Dihydrofolate reductase (DHFR) is a key and essential enzyme in the folate pathway that converts dihydrofolate (DHF) to tetrahydrofolate (THF) (Raimondi et al., 2019). This coenzyme is required for a variety of cellular processes, including the synthesis of purine involved in nucleic acid and amino-acid biosynthesis. The active site is located in a cleft formed by α-helix 1, α-helix 2, α-helix 4 and β-sheet 1, similar to CglDHFR and CalDHFR. As classified in E. coli DHFR, CauDHFR could also be designated to have two subdomains: the nucleotide subdomain, in which the NADPH sits, and the substrate-binding subdomain, which is predominantly formed by α-helix 1, α-helix 2 and β-sheet 1.

Crystals of apo and holo CauDHFR have a single protomer in the asymmetric unit, while the ternary complexes CauDHFR–NADPH–PYR and CauDHFR–NADPH–CYG contained two protein molecules which are independent and do not form a quaternary structure, according to the PISA server. In order to obtain the structures of the CauDHFR–NADPH–PYR and CauDHFR–NADPH–CYG ternary complexes, the N-terminal His tag of the protein needed to be removed since analysis of the crystal packing of the CauDHFR–NADPH complex showed that the N-terminus of the adjacent symmetric protomer extends into the substrate-binding site, blocking ligand access. The NADPH binding site is located in a very positively charged cleft between α-helix 2 and α-helix 4, in which the cofactor is involved in an extensive number of hydrogen-bonding interactions. The diphosphate groups interact with both α-helix 2 and α-helix 4, specifically with Gly54, Thr57, Gly122, Ser123 and Gln124. The adenine group interacts with Leu76, Ser77, Arg78 and Leu128 between α-helix 3 and α-helix 4, which is the most solvent-exposed moiety of NADPH. The ribose ring makes interactions with Ile19, Gly23 and Ser24 from the substrate-binding domain, which is the most neutral region of the cofactor-binding site. The nicotinamide moiety is buried in the active site of the enzyme, interacting with Ala11, Ile19, Leu25 and Tyr126, extending further towards the substrate-binding subdomain. The substrate-binding regions of apo and holo CauDHFR are largely similar, with the addition of NADPH not making a substantial difference to most residue orientations. The main difference observed is movement of Leu25, with a change of 5 Å between the isopropyl functional groups.

> GLVPRGSHMMSTRPKISLIVAALQPSMGIGAKGSLPWRLKNEMKYFKDVTSKAKDGHINAVVMGRKTWELIPERFRPLAGRLNVILSRKNDDLIDSNGVYHFSSFDSVMKHLEKDSFRFKDMPLDKIFIIGGSQIYNLLILDSRVDNLLVTQVHFVGEDADKPQMDTFLDWDLSKWKRLEHDKLEQYVGLDVPRGLNEEGSYNYEYTMWEKAQ> MIEIKDKQLTGLRFIDLFAGLGGFRLALESCGAECVYSNEWDKYAQEVYEMNFGEKPEGDITQVNEKT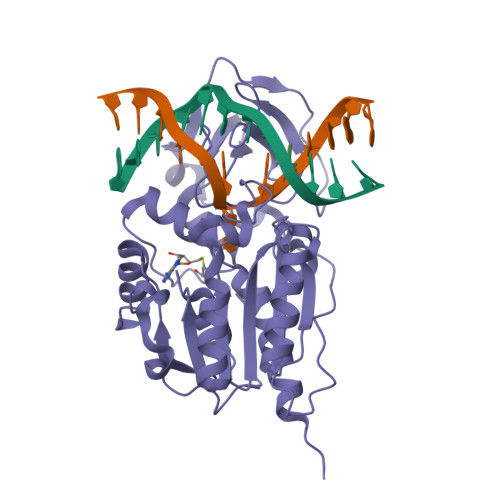IPDHDILCAGFPCQAFSISGKQKGFEDSRGTLFFDIARIVREKKPKVVFMQNVKNFASHDNGNTLEVVKNTMNELDYSFHAKVLNALDYGIPQKRERIYMICFRNDLNIQNFQFPKPFELNTFVKDLLLPDSEVEHLVIDRKDLVMTNQEIEQTTPKTVRLGIVGKGGQGERIYSTRGIAITLSAYGGGIFAKTGGYLVNGKTRKLHPRECARVMGYPDSYKVHPSTSQAYKQFGNSVVINVLQYIAYNIGSSLNFKPY>MASWSHPQFEKMGMLEARELLCERDERTLFSGLSFTLNAGEWVQITGSNGAGKTTLLRLLTGLSRPDAGEVLWQGQPLHQVRDSYHQNLLWIGHQPGIKTRLTALENLHFYHRDGDTAQCLEALAQAGLAGFEDIPVNQLSAGQQRRVALARLWLTRATLWILDQPFTAIDVNGVDRLTQRMAQHTEQGGIVILTTHQPLNVAESKIRRISLTQTRAA[2x];>MMFWRIFRLELRVAFRHSAEIANPLWFFLIVITLFPLSIGPEPQLLARIAPGIIWVAALLSSLLALERLFRDDLQDGSLEQLMLLPLPLPAVVLAKVMAHWMVTGLPLLILSPLVAMLLGMDVYGWQVMALTLLLGTPTLGFLGAPGVALTVGLKRGGVLLSILVLPLTIPLLIFATAAMDAASMHLPVDGYLAILGALLAGTATLSPFATAAALRISIQ[2x];> MWKTLHQLAIPPRLYQICGWFIPWLAIASVVVLTVGWIWGFGFAPADYQQGNSYRIIYLHVPAAIWSMGIYASMAVAAFIGLVWQMKMANLAVAAMAPIGAVFTFIALVTGSAWGKPMWGTWWVWDARLTSELVLLFLYVGVIALWHAFDDRRLAGRAAGILVLIGVVNLPIIHYSVEWWNTLHQGSTRMQQSIDPAMRSPLRWSIFGFLLLSATLTLMRMRNLILLMEKRRPWVSELILKRGRK;> MTPAFASWNEFFAMGGYAFFV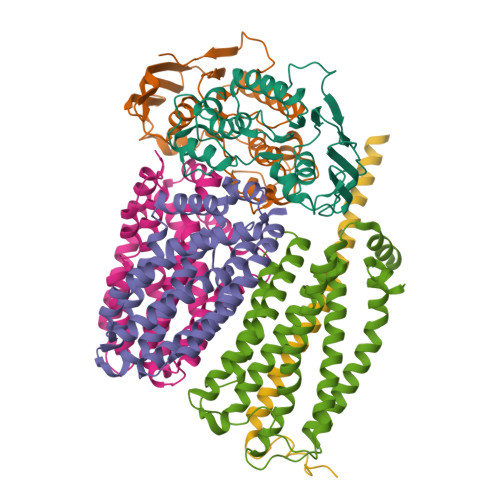WLAVVMTVIPLVVLVVHSVMQHRAILRGVAQQRAREARLRAAQQQEAA>[10x]MTKFYSPDDLVTPQEFADPHFAAINQKRFDLYIDLRVQGYSSWRVFRAIWGEEHMDGPAQARIFAMESNPYYRKQFKAKLNATKTSDLWNPKTALHELL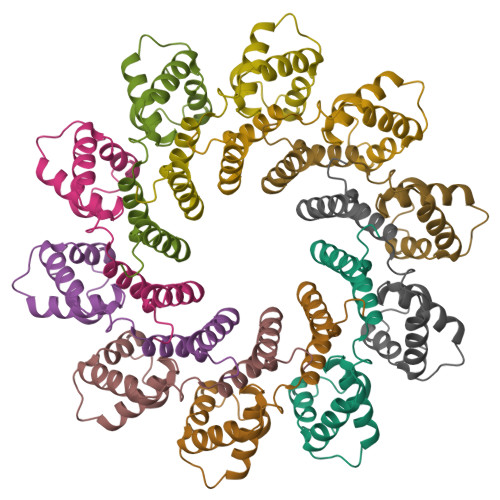QMVRDPTVKDSSRLSAIKELNVLAEITFVDESGKTRIGRGLADFYASEAEAQTATVAAAAEANSYVPEGEEGDFPSPTPEPTEEDRANPI The serine/threonine protein kinase AKT plays a pivotal role within the PI3K pathway in regulating cellular proliferation and apoptotic cellular functions, and AKT hyper-activation via gene amplification and/or mutation has been implicated in multiple human malignancies. AKT is a serine/threonine kinase which plays a key role in the phosphatidylinositol-3-kinase (PI3K)/AKT/mammalian target of rapamycin (mTOR) signalling pathway and is involved in cell signalling, proliferation, glucose metabolism and protein synthesis via phosphorylation of two critical residues, threonine 308 and serine 4731,2. Small molecule AKT inhibitors are typically either ATP competitive or allosteric with respect to their binding site. Allosteric inhibitors induce a conformational change through binding to the pleckstrin homology (PH) domain, thus preventing localisation of AKT to the plasma membrane and therefore inhibiting activation of the pathway.

We present the discovery and development of ALM301, a novel, allosteric, sub-type selective inhibitor of AKT1/2. The allosteric binding mode of this series was confirmed via a high resolution (2.32 Å) co-crystal structure obtained with a close analogue of ALM301 (compound 3) in complex with AKT2. Compound 3 binds in an allosteric binding pocket ca. 10 Å away from the hinge backbone (dark blue) at the interface of the N- and C-lobes of the kinase and PH domains, similar to previously published allosteric AKT inhibitors. The crystal structure showed compound 3 binding to a DFG-out conformation of AKT2, restricting access to the ATP binding site. ALM301 adopted a similar binding mode to compound 3 when docked into the compound 3 binding site. The bicyclic moiety of ALM301 was predicted to stack against Trp80 with the carbonyl group close to the Arg209 sidechain but not forming a direct hydrogen bond. The unsubstituted phenyl ring occupies the hydrophobic pocked under the DFG loop that would be occupied by Phe294 when the protein adopts a DFG-in conformation. The docked pose places the para-substituted phenyl pointing towards the catalytic subunit, with the polar substituents both forming interactions with the protein; the basic nitrogen forms a salt bridge with Asp275, and the hydroxyl a hydrogen bond with the Glu299 sidechain. ALM301 binds in an allosteric pocket created by the combined movement of the PH domain and the catalytic domain, resulting in a DFG out conformation. Incubating ALM301 with increasing concentrations of ATP had no effect on the biochemical IC50 value versus AKT1, confirming that the mode of binding for ALM301 is allosteric and independent of ATP concentration.

> GAMDEVSVIKEGWLHKRGEYIKTWRPRYFLLKSDGSFIGYKERPEAPDQTLPPLNNFSVAECQLMKTERPRPNTFVIRCLQWTTVIERTFHVDSPDEREEWMRAIQMVANSLKQRAPGEDPMDYKCGSPSDSSTTEEMEVAVSKARAKVTMNDFDYLKLLGKGTFGKVILVREKATGRYYAMKILRKEVIIAKDEVAHTVTESRVLQNTRHPFLTALKYAFQTHDRLCFVMEYANGGELFFHLSRERVFTEERARFYGAEIVSALEYLHSRDVVYRDIKLENLMLDKDGHIKITDFGLCKEGISDGATMKTFCGTPEYLAPEVLEDNDYGRAVDWWGLGVVMYEMMCGRLPFYNQDHERLFELILMEEIRFPRTLSPEAKSLLAGLLKKDPKQRLGGGPSDAKEVMEHRFFLSINWQDVVQKKLLPPFKPQVTSEVDTRYFDDEFTAQSITITPPDRYDSLGLLELDQRTHFPQFSYSASIRE>SHMDVKGALFMNGGDLESSYAQHGCFSQKVTSITKPILVNAIHSLFSEYFHREKVLNVADLGCAAGPNPFSVILTVKESLERKCKELNCQPAELQVYLNDLPGNDFNSLFKDLSGVGKDQKSDVLRTCFVMGAPGSFYGRLFPRSCLHLVHSCYSVHWLSQVPKGLTSKEGLPLNKGKINISKTSPPVVEAAYLAQFKEDFTLLLKSRAEEMVQNGRMVLILNGRQASDPWGKESCYHWEVLAEAISEMVSQGLVDEEKLDSFNVPCYAPSQEEVQDIVDKVGSFAVEHIETFTLPFANDQESDTRVKGEQLAKNIRSFTESIISYEFGKEITEKVYHKLTQIVVKDMASRPPTNTTVVVVLSRTM[2x]

Our phylogenetic analysis showed that although the YM genome does not appear to encode XMT-type caffeine-producing enzymes like Coffea and Citrus, it does contain three recently and tandemly duplicated genes that encode CS-type enzymes, IpCS1, IpCS2, and IpCS3. A second enzyme, IpCS2, shows activity only with 3X to produce TB, while a third enzyme, IpCS3, exhibits a preference to methylate TB to form CF. Thus, collectively, these three enzymes appear capable of catalysing a complete pathway from xanthine to caffeine.

In order to gain insight into the structural basis for the convergent enzyme activities, we obtained a crystal structure for the terminal enzyme in the pathway that forms caffeine. As is typical for the SABATH family of methyltransferases, IpCS3 exhibits a Rossman-like fold composed of seven β-strands surrounded by five α-helices which bind the methyl-donor S-adenosyl-L-methionine (SAM), as well as an α-helical cap which binds the methyl-acceptor theobromine. Although the IpCS3 structure was obtained in complex with its product, caffeine, it can be assumed that the binding mode is conserved for its precursor, theobromine. Indeed, our computational modelling of theobromine in the active site of IpCS3 predicts it to be oriented as we have discerned from the diffraction data. In CcDXMT, the NE2 of His160 and NE1 of Trp161 form hydrogen bonds to carbonyl O2 of TB when positioned for N1 methylation; yet, in the structure of IpCS3 these corresponding side chain groups form hydrogen bonds to O6 of TB. Despite these two residues being conserved for H-bonding, the substrates are rotated 180° along an axis going through N1 and C4. Thus, the conserved His and Trp residues interact with opposing carbonyls in TB/CF but still position the substrate for N1 methylation. Tyr368 of CcDXMT is found to participate in π–π interactions with the ring structure of TB Lanzarotti et al., 2020; yet in IpCS3, Asn353 is found in the homologous position and the amine forms a hydrogen bond with N9 due to its proximity within 3.2 Å, which is additionally stabilized by Asn221 and His236. Because the residues in these positions of IpCS3 and CcDXMT differ yet contribute to TB binding, these independent replacements represent convergent structural solutions for N1 methylation of the substrate.4-(DIMETHYLAMINO)BUTYL 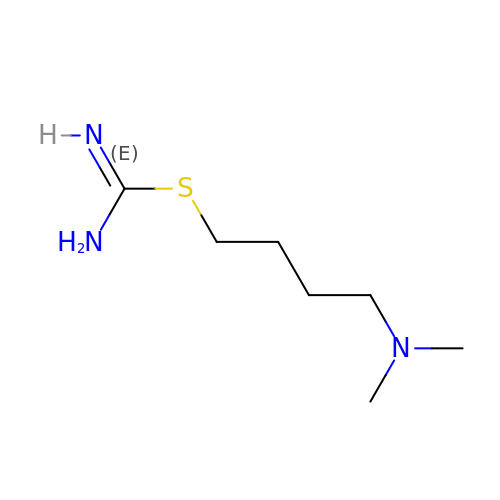IMIDOTHIOCARBAMATE | C7 H17 N3 S | UFYJLJINUGVUHO-UHFFFAOYSA-N The APL1 proteins contain a signal peptide, a leucine-rich repeat (LRR) domain and a cysteine-rich region followed by a C-terminal coiled-coil (CC) domain containing a helix-loop-helix (HLH) motif. LRIM1 and APL1A—C are members of an LRR family, the LRIM family, that includes several dozen genes found within, but not outside, mosquito genomes (family Culicidae) and are believed to play multiple roles within the innate immune system. The APL1 genes are homologous in sequence, polymorphic and under positive selection pressure. Structural analysis of APL1B identified that the protein exists as a homodimer that is mediated by a unique N-terminus which has no homology to other LRIM family members.

To determine the molecular basis of APL1B-LRR homodimerization, we crystallized APL1B-LRR and solved the structure to 1.74 Å resolution. The refined model contains two molecules of APL1B-LRR in the asymmetric unit, residues 25–364 for chain A and residues 27–364 for chain B (the crystallized protein comprises APL1B 21–370 and a C-terminal 6×His tag). Of the three predicted N-linked glycosylation sites (Asn166, Asn211, Asn317) a single N-acetylglucosamine was resolved for residue Asn166 of each domain. The overall structure of APL1B-LRR is similar to APL1C-LRR (Cα rmsd 0.605 Å). However, APL1B has two fewer LRRs than APL1C so the overall length of its LRR domain is ~70 Å versus ~80 Å for APL1C. A homodimeric interface exists between the two APL1B-LRR domains in the asymmetric unit that buries an area of ~1500 Å2 representing 9–10% of total solvent-accessible surface area. The dimer interface is formed between the N-terminal helix of one domain and the first LRR of the other domain. The two N-terminal helices form a dovetail joint between the solenoid LRRs that hold the two domains at a 90° angle to each other. Residues 31–44 form an amphipathic α-helix such that Leu35, Leu38, Leu39, and Phe42 pack against the first LRR, protecting the hydrophobic surface from the solvent. Interestingly, a short, well resolved β-strand on the N-terminal loop of one domain (Met28–Leu30) forms a parallel β-sheet with a β-strand on the first LRR of the second domain (Ile55–Ile58).

>[2x]GQLSYKSMHLTPFTLSALLASFHKVEVLNLNGLQIEEIDTNAFAYAHTIQKLYMRFNVIRYLPPHVFQNVPLLTVLMLDRNDLSSLPPGIFHNTPKLTMMSMSNNNLERIEDDTFQATTALQNLQLSSNRLTHVDLALIPSLFHVNVSYNLLSTLAIPIAVEELDASHNTINVVRGPVNVELTILKLQHNNLTDTAWLLNYPGLVDVDLSYNQLEKITYQHFVKMQRLERLYVSNNRLVALDFYGRPIPTLKVLDLSHNHLMWVEHNQAQFDKLQYLYLDHNSIVTFKLSTSHTLKNLTLSHNDWDCNSLRALFRNVAQPAVHDADQHCKIDYHLEHGLCCKESDKPYLDHHHHHH> MSGEKIDITPKKDGGVLKLIKKEGQGVVKPTTGTTVKVHYVGTLENGTKFDSSRDRGDQFSFNLGRGNVIKGWDLGVATMTKGEVAEFTI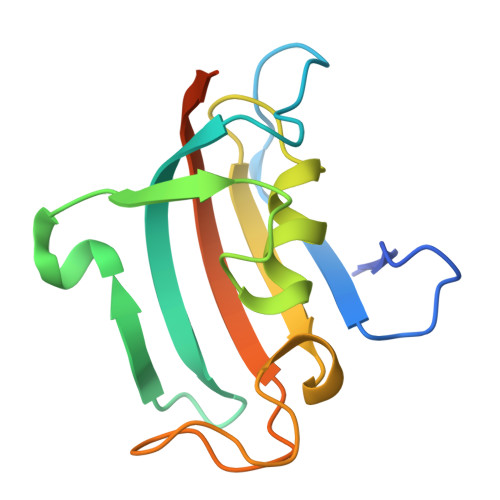RSDYGYGDAGSPPKIPGGATLIFEVELFEWSAEDISPDRDGTILR> GPHMEEIMQSDSKIEKMLPDGGRLVVFPNGTRKELSADGQTVKVMFFNGDVKHTMPDQRVIYYYAEAQTTHITYPDGMEVLQFPNNQTEKHFPDGRKEITFPDQTVKTLHPDGREESVLTDGTIIQLNPDGSKVIQFN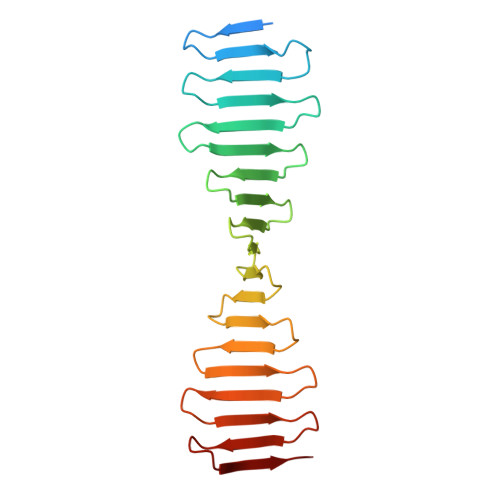TGQREIHTADFKRREYPDGTVKTVYSDGRQETQYPTGRVRLKDPQGKVIMDTKA> MPKEKPHV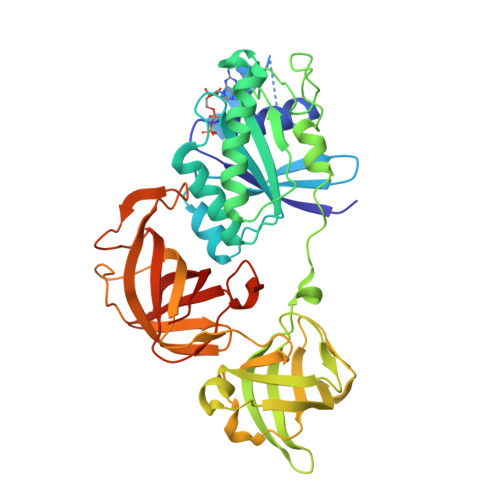NIVFIGHVDHGKSTTIGRLLYDTGNIPETIIKKFEEMGEKGKSFKFAWVMDRLKEERERGITIDVAHTKFETPHRYITIIDAPGHRDFVKNMITGASQADAAVLVVAATDGVMPQTKEHAFLARTLGIKHIIVTINKMDMVNYDQKVFEKVKAQVEKLLKTLGYKDFPVIPTSAWNGDNVVKKSDKMPWYNGPTLIEALDQIPEPEKPIDKPLRIPIQDVYSIKGVGTVPVGRVETGKLKVGDVVIFEPASTIFHKPIQGEVKSIEMHHEPLQEALPGDNIGFNVRGVSKNDIKRGDVAGHTDKPPTVVRTKDTFKAQIIVLNHPTAITVGYSPVLHAHTAQIPVRFEQILAKVDPRTGNIVEENPQFIKTGDSAIVVLRPMKPVVLEPVKEIPQLGRFAIRDMGMTIAAGMVISIQKGEHHHHHH> MKTLVHVASVEKGRSYEDFQKVYNAIALKLREDDEYDNYIGYGPVLVRLAWHISGTWDKHDNTGGSYGGTYRFKKEFNDPSNAGLQNGFKFLEPIHKEFPWISSGDLFSLGGVTAVQEMQ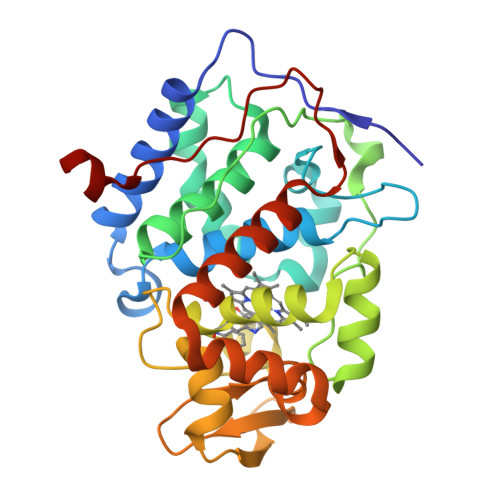GPKIPWRCGRVDTPEDTTPDNGRLPDADKDAGYVRTFFQRLNMNDREVVALMGAHALGKTHLKNSGYEGPGGAANNVFTNEFYLNLLNEDWKLEKNDANNEQWDSKSGYMMLPTDYSLIQDPKYLSIVKEYANDQDKFFKDFSKAFEKLLENGITFPKDAPSPFIFKTLEEQGL Crystal structures of THAS (here referred to as THAS1), a second representative THAS (Cr_021691, THAS2) and the structure of the promiscuous homologue (Cr_032583b, HYS) were solved and mutants revealed key residues that control the stereochemistry of the product profiles. The HYSs perform a single, chemically straightforward reduction reaction that immediately neutralizes the reactivity of strictosidine aglycone/cathenamine. The biological unit is an elongated homodimer, with each subunit divided into a substrate and cofactor-binding domain; the latter also being responsible for forming the dimer interface. The active site cavities of the HYSs are framed by helix α2, the catalytic zinc coordination sphere, and loops 1 and 2, with the NADP(H) co-substrate binding at the base of the active site.

We recently reported the first cloning of a biosynthetic gene encoding an enzyme that acts on strictosidine aglycone. This zinc-dependent medium chain dehydrogenase/reductase (MDR), named tetrahydroalstonine synthase (THAS), produces the heteroyohimbine tetrahydroalstonine. THAS1 and THAS2, which produce predominantly tetrahydroalstonine, were both crystallized, since their amino acid sequence identity is relatively low (55%) and the predicted active sites have numerous differences. Structures were obtained for THAS1 and THAS2 with NADP+ bound (THAS1, 1.05 Å resolution; THAS2, 2.10 Å resolution) and in apo form (THAS1, 2.25 Å resolution; THAS2, 2.05 Å resolution), while HYS could only be crystallized in the apo form (2.25 Å resolution). Interestingly, a non-proline cis-peptide is present in the THAS1-NADP+ and HYS apo structures. Closer inspection of this region in THAS1 shows that when this bond is in the trans conformation, the side chain of Asp340 is projected into the cofactor-binding site such that it would prevent NADPH binding. SAD/CAD utilize an active site serine that protonates the alkoxide that results from reduction of the aldehyde substrate; this serine is replaced with a tyrosine residue in THAS1 (Tyr56) and HYS (Tyr53). Mutation of other conserved ionizable residues in the THAS1 active site (Tyr56, Ser102 and Thr166) did not result in substantial changes in the distribution of products. Mutations to Glu59, which anchors the NADPH cofactor, resulted in a slight increase in product promiscuity, perhaps by causing a shift in the cofactor position.

>GPAMASKSPSEEVYPVKAFGLAAKDSSGLFSPFNFSRRATGEHDVQLKVLYCGTCQYDREMSKNKFGFTSYPYVLGHEIVGEVTEVGSKVQKFKVGDKVGVASIIETCGKCEMCTNEVENYCPEAGSIDSNYGACSNIAVINENFVIRWPENLPLDSGVPLLCAGITAYSPMKRYGLDKPGKRIGIAGLGGLGHVALRFAKAFGAKVTVISSSLKKKREAFEKFGADSFLVSSNPEEMQGAAGTLDGIIDTIPGNHSLEPLLALLKPLGKLIILGAPEMPFEVPAPSLLMGGKVMAASTAGSMKEIQEMIEFAAEHNIVADVEVISIDYVNTAMERLDNSDVRYRFVIDIGNTLKSN[2x]>MASTRCKLARYLEDLEDVDLKKFKMHLEDYPPQKGCIPLPRGQTEKADHVDLATLMIDFNGEEKAWAMAVWIFAAINRRDLYEKAKRDEPKWGSDNARVSNPTVICQE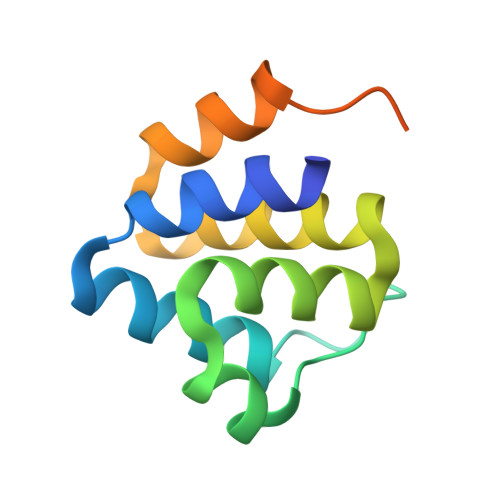DS[2x]>PVNPCCYYPCQHQGICVRFGLDRYQCDCTRTGYSGPNCTIPEIWTWLRTTLRPSPSFIHFLLTHGRWLWDFVNATFIRDTLMRLVLTVRSNLIPSPPTYNIAHDYISWESFSNVSYYTRILPSVPRDCPTPMGTKGKKQLPDAEFLSRRFLLRRKFIPDPQGTNLMFAFFAQHFTHQFFKTSGKMGPGFTKALGHGVDLGHIYGDNLERQYQLRLFKDGKLKYQMLNGEVYPPSVEEAPVLMHYPRGIPPQSQMAVGQEVFGLLPGLMLYATIWLREHNRVCDLLKAEHPTWGDEQLFQTARLILIGETIKIVIEEYVQQLSGYFLQLKFDPELLFGAQFQYRNRIAME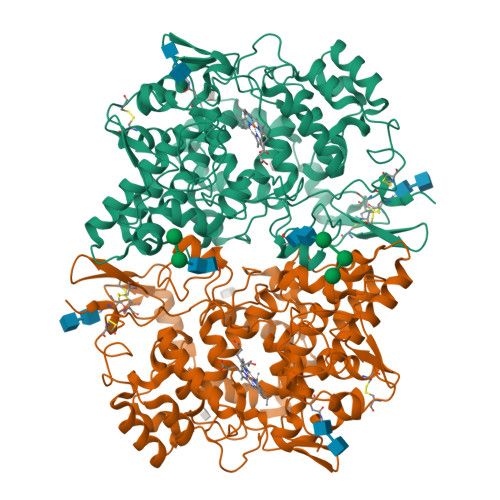FNQLYHWHPLMPDSFRVGPQDYSYEQFLFNTSMLVDYGVEALVDAFSRQPAGRIGGGRNIDHHILHVAVDVIKESRVLRLQPFNEYRKRFGMKPYTSFQELTGEKEMAAELEELYGDIDALEFYPGLLLEKCHPNSIFGESMIEMGAPFSLKGLLGNPICSPEYWKASTFGGEVGFNLVKTATLKKLVCLNTKTCPYVSFHVPD[2x]>ADTIVAVELDTYPNTDIGDPSYPHIGIDIKSVRSKKTAKWNMQNGKVGTAHIIYNSVGKRLSAVVSYPNGDSATVSYDVDLDNVLPEWVRVGLSASTGLYKETNTILSWSFTSKLKSNSTHETNALHFVFNQFSKDQKDLILQGDATTGTDGNLELTRVSSNGSPQGSSVGRALFYAPVHIWESSAVVASFDATFTFLIKSPDSHPADGIAFFISNIDSSIPSGSTG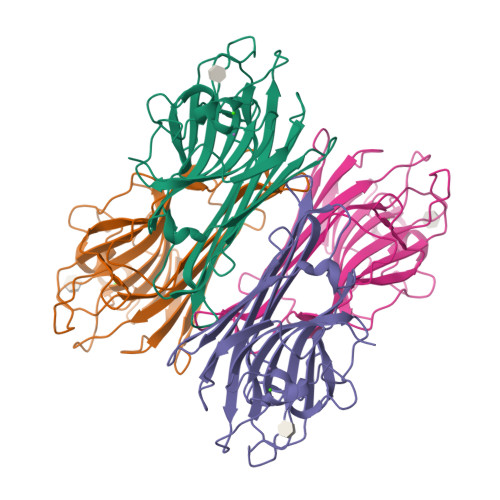RLLGLFPDAN[2x]(1S,3R,4S)-3-formyl-4-[({3-hydroxy-2-methyl-5-[(phosphonooxy)methyl]pyridin-4-yl}methyl)amino]cyclopentane-1-carboxylic acid | C15 H21 N2 O8 P | 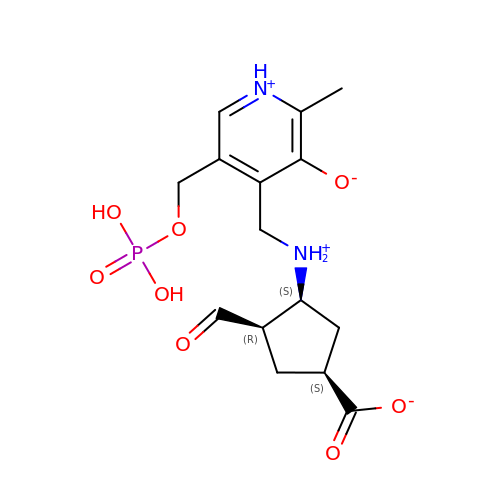QPJGRJWUQOEMOU-KWBADKCTSA-N>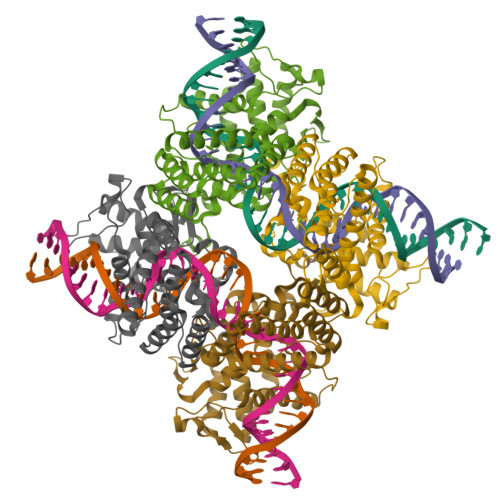[4x]MSNLLTVHQNLPALPVDATSDEVRKNLMDMFRDRQAFSEHTWKMLLSVCRSWAAWCKLNNRKWFPAEPEDVRDYLLYLQARGLAVKTIQQHLGQLNMLHRRSGLPRPSDSNAVSLVMRRIRKENVDAGERAKQALAFERTDFDQVRSLMENSDRCQDIRNLAFLGIAYNTLLRIAEIARIRVKDISRTDGGRMLIHIGRTATLVSTAGVEKALSLGVTKLVERWISVSGVADDPNNYLFCRVRKNGVAAPSATSQLSTRALEGIFEATHRLIYGAKDDSGQRYLAWSGHSARVGAARDMARAGVSIPEIMQAGGWTNVNIVMNYIRNLDSETGAMVRLLEDGD>SSPGKPPRLVGGPMDASVEEEGVRRALDFAVGEYNKASNDMYHSRALQVVRARKQIVAGVNYFLDVELGRTTCTKTQPNLDNCPFHDQPHLKRKAFCSFQIYAVPWQGTMTLSK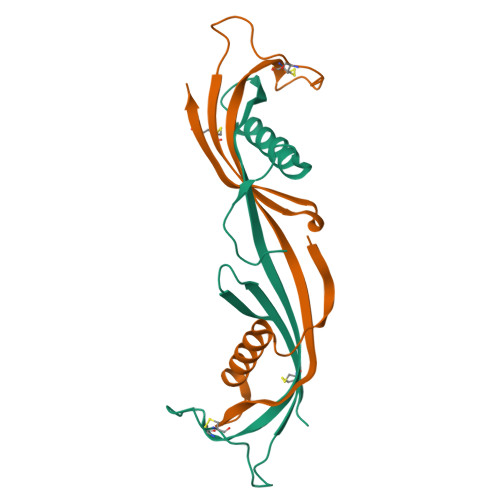STCQDA[2x]>[2x]TQKPSLYRVLILNDDYTPMEFVVYVLERF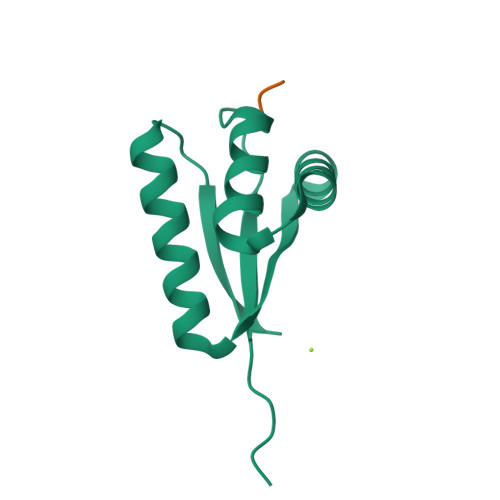FNKSREDATRIMLHVHQNGVGVCGVYTYEVAETKVAQVIDSARRHQHPLQCTMEKD;>WLFVQRDSKE[2x]> GGMAQVSKQTSKKRELSIDEYQGARKWCFTIAFNKALVNRDKNDGLFVESLLRHEKYSKHDWYDEDTRALIKCSTQAANAKAEALANYFSAYRHSPGCLTFTAEDELRTIMERAYERAIFECRRRETEVI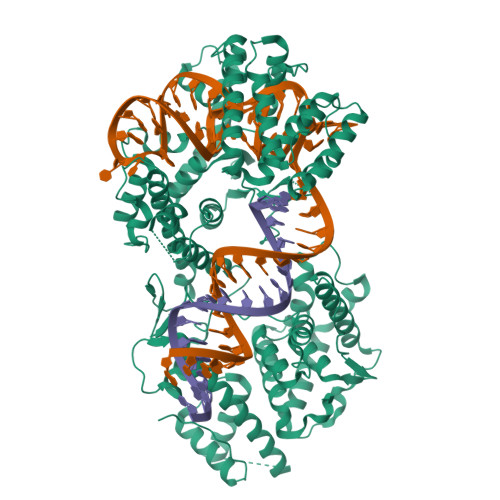IEFPSLFEGDRITTAGVVFFVSFFVERRVLDRLYGAVSGLKKNEGQYKLTRKALSMYCLKDSRFTKAWDKRVLLFRDILAQLGRIPAEAYEYYHGEQGDKKRANDNEGTNPKRHKDKFIEFALHYLEAQHSEICFGRRHIVREEAGAGDEHKKHRTKGKVVVDFSKKDEDQSYYISKNNVIVRIDKNAGPRSYRMGLNELKYLVLLSLQGKGDDAIAKLYRYRQHVENILDVVKVTDKDNHVFLPRFVLEQHGIGRKAFKQRIDGRVKHVRGVWEKKKAATNEMTLHEKARDILQYVNENCTRSFNPGEYNRLLVCLVGKDVENFQAGLKRLQLAERIDGRVYSIFAQTSTINEMHQVVCDQILNRLCRIGDQKLYDYVGLGKKDEIDYKQKVAWFKEHISIRRGFLRKKFWYDSKKGFAKLVEEHLESGGGQRDVGLDKKYYHIDAIGRFEGANPALYETLARDRLCLMMAQYFLGSVRKELGNKIVWSNDSIELPVEGSVGNEKSIVFSVSDYGKLYVLDDAEFLGRICEYFMPHEKGKIRYHTVYEKGFRAYNDLQKKCVEAVLAFEEKVVKAKKMSEKEGAHYIDFREILAQTMCKEAEKTAVNKVARAFFAHHLKFVIDEFGLFSDVMKKYGIEKEWKFPVK>MKAAVVNEFKKALEIKEVERPKLEEGEVLVKIEACGVCHTDLHAAHGDWPIKPKLPLIPGHEGVGIVVEVAKGVKSIKVGDRVGIPWLYSACGECEYCLTGQETLCPHQLNGGYSVDGGYAEYCKAPADYVAKIPDNLDPVEVAPILCAGVTTYKALKVSGARPGEWVAIYGIGGLGHIALQYAKAMGLNVVAVDISDEKSKLAKDLGADIAINGLKEDPVKAIHDQVGGVHAAISVAVNKKAFEQAYQSVKRGGTLVVVGLPNADLPIPIFDTVLNGVSVKGSIVGTRKDMQEALDFAA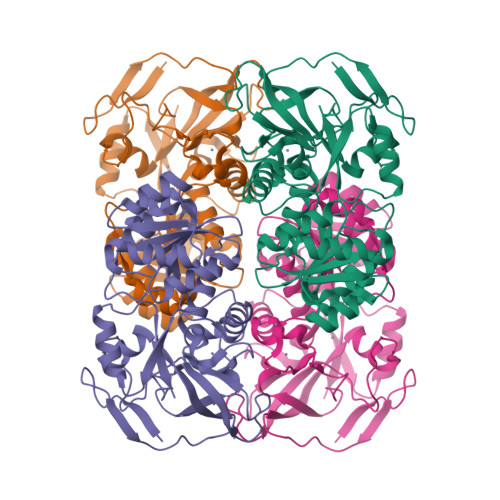RGKVRPIVETAELEEINEVFERMEKGKINGRIVLKLKED[8x]> GVTKNNSCKKVGVEELINEKGCDLMIIRINRCRGHCFSFTFPNPLTKKYSVHAKCCRMVEWEMLETELKCSKGNRNLRIPSATQCECFDCLV;> GKECEFAMRLVPGFNPLRQVDANGKECRGNVELPFCKGYCKTSESGTHGFPPRVQNSKVCTLVTTSTRKVVLDDCDDGADESVKFVMVPHGTDCECSAV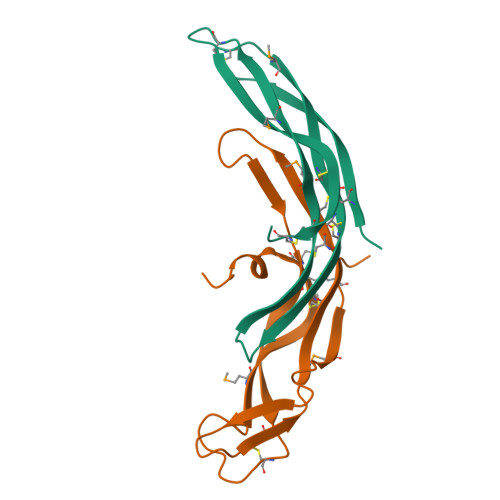PLEQHHS1,5-diphenyl-N-(1H-tetrazol-5-yl)-1H-pyrazole-3-carboxamide | C17 H13 N7 O | 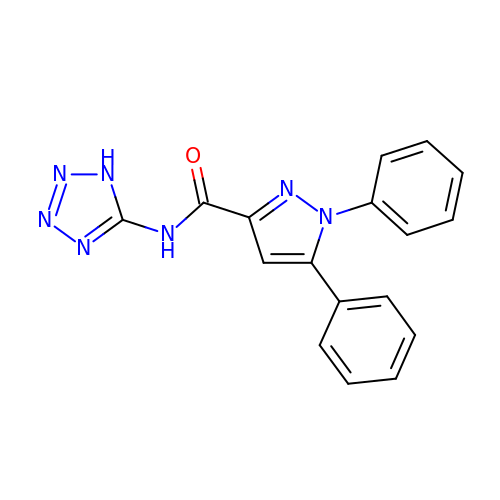QVLVNOAMAMUIJM-UHFFFAOYSA-N>MTQKFGLSAALTTP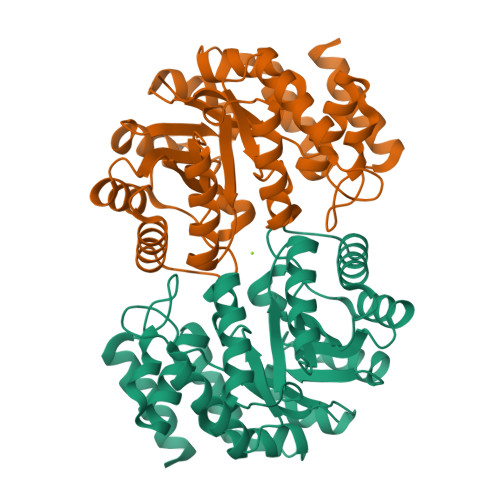FKTDGTVDIDAMIAHARRCLSNGCDSVTLFGTTGEGCSVGSRERQAILSSFIAAGIAPSRIVTGVLVDSIEDAADQSAEALNAGARNILLAPPSYFKNVSDDGLFAWFSAVFSKIGKDARDILVYNIPSVTMVTLSVELVGRLKAAFPGIVTGVKDSSGNWSHTERLLKEHGDLAILIGDERDLARGVRLGGQGAISGVANFLTQEVRAMAVDGKDDPRIVDLVVELLKFPVTPAVKVLVSHTTGETIWSDVRAPLVAISPEDRRQIEGAFDALFRRQAA[2x]> MAHHHHHHHMNVVFVGAEMAPWSKTGGLGDVLGGLPPAMAANGHRVMVISPRYDQYKDAWDTSVVAEIKVADRYERVRFFHCYKRGVDRVFIDHPSFLEKVWGKTGEKIYGPDTGVDYKDNQMRFSLLCQAALEAPRILNLNNNPYFKGTYGEDVVFVCNDWHTGPLASYLKNNYQPNGIYRNAKVAFCIHNISYQGRFAFEDYPELNLSERFRSSFDFIDGYDTPVEGRKINWMKAGILEADRVLTVSPYYAEELISGIARGCELDNIMRLTGITGIVNGMDVSEWDPSKDKYITAKYDATTAIEAKALNKEALQAEAGLPVDRKIPLIAFIGRLEEQKGPDVMAAAIPELMQEDVQIVLLGTGKKKFEKLLKSMEEKYPGKVRAVVKFNAPLAHLIMAGADVLAVPSRFEPCGLIQLQGMRYGTPCACASTGGLVDTVIEGKTGFHMGRLSVDCKVVEPSDVKKVAATLKRAIKVVGTPAYEEMVRNCMNQDLSWKGPAKNWENVLLGLGVAGSAPGIEGDEIA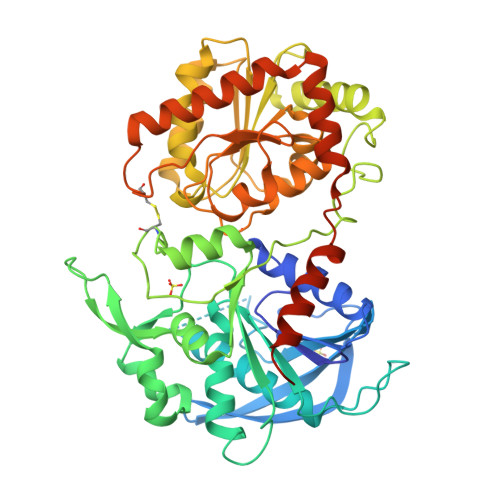PLAKENVAAP> MTDLSPLQTRVEAGIAWLVLNRPQQRNALDIPTLEALHVRLDACERDPAVRAVVLGGSGRSFCAGADLAEWAAAEARGELESYGWTEAAHALMGRLHALDKPTVAAVNGSAVGAGMDLALCCDFRIAAAS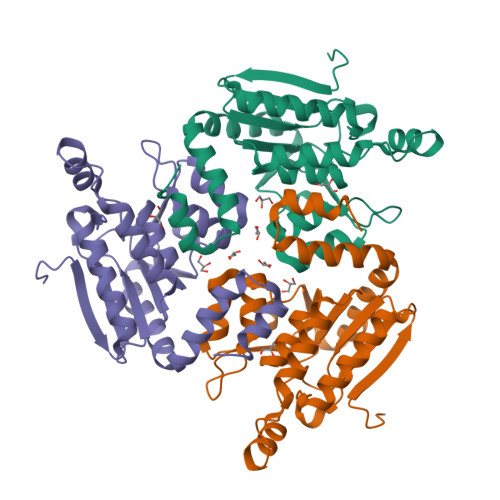ARFKAGYTGMAYCPDAGASWHLPRLLGSEAAKRLLFLDEAWSAERALGAGLVGEVVADEHLVEAVGAFAARLASGPTFAFAQTKRLLRDGAGRSLAEQLRAEQAAGLLCGRSEDAAEALRAVAEKRSPQFSGRLEHHHHHH>MASWKGLIHQYKEFLPVTDQTPALTLHEGNTPLIHLPKLSEQLGIELHVKTEGVNPTGSFKDRGMVMAVAKAKEEGNDTIMCASTGNTSAAAAAYAARANMKCIVIIPNGKIAFGKLAQAVMYGAEIIAIDGNFDDALKIVRSICEKSPIALVNSVNPYRLEGQKTAAFEVCEQLGEAPDVLAIPVGNAGNISAYWKGFKEYHEKNGTSLPKMRGFEAEGSAAIVRNEVIENPETIATAIRIGNPASWDKAVKAAEESNGKIDEVTDDEILHAYQLIAREEGVFAEPGSCASIAGVLKQVKSGEIPKGSKVVAVLTGNGLKDPNTAVDISEIKPVTLPTNEDSILEYVKGAAR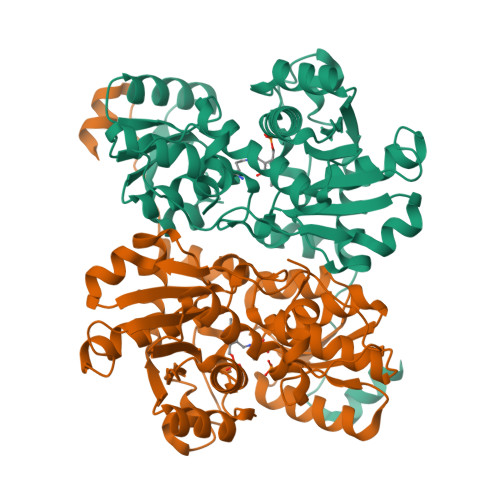V[2x]>[2x]SNAMTGTLLSFGHGYTARVLSRALAPQGWRIIGTSRNPDQMEAIRASGAEPLLWPGEEPSLDGVTHLLISTAPDSGGDPVLAALGDQIAARAAQFRWVGYLSTTAVYGDHDGAWVDETTPLTPTAARGRWRVMAEQQWQAVPNLPLHVFRLAGIYGPGRGPFSKLGKGGIRRIIKPGQVFSRIHVEDIAQVLAASMARPDPGAVYNVCDDEPV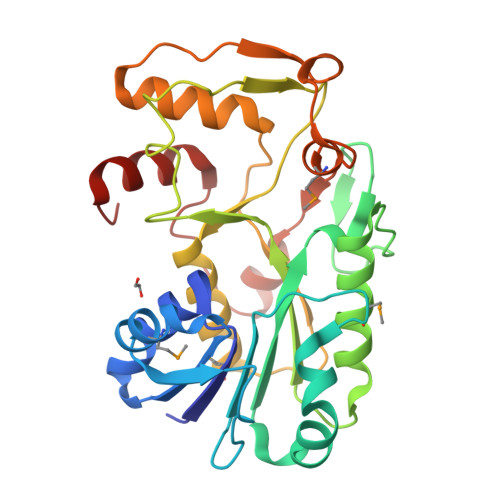PPQDVIAYAAELQGLPLPPAVDFDKADLTPMARSFYSENKRVRNDRIKEELGVRLKYPNYRVGLEALQADAET> GSHMLSDEQMQIINSLVEAHHKTYDDSYSDFVRFRPPVREGPVTRSASRAASLHSLSDASSDSFNHSPESVDTKLNFSNLLMMYQDSGSPDSSEEDQQSRLSMLPHLADLVSYSIQKVIGFAKMIPGFRDLTAEDQIALLKSSAIEIIMLRSNQSFSLEDMSWSCGGPDFKYCINDVTKAGHTLELLEPLVKFQVGLKKLKL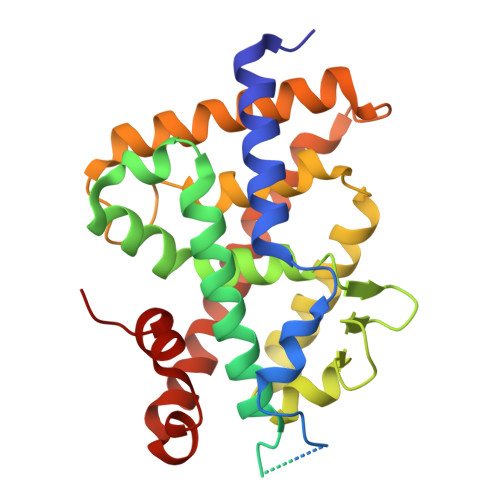HEEEHVLLMAICLLSPDRPGVQDHVRIEALQDRLCDVLQAYIRIQHPGGRLLYAKMIQKLADLRSLNEEHSKQYRSLSFQPEHSMQLTPLVLEVFGSEVS>PFLELDTNLPANRVPAGLEKRLCAAAASILGKPADRVNVTVRPGLAMALSGSTEPCAQLSISSIGVVGTAEDNRSHSAHF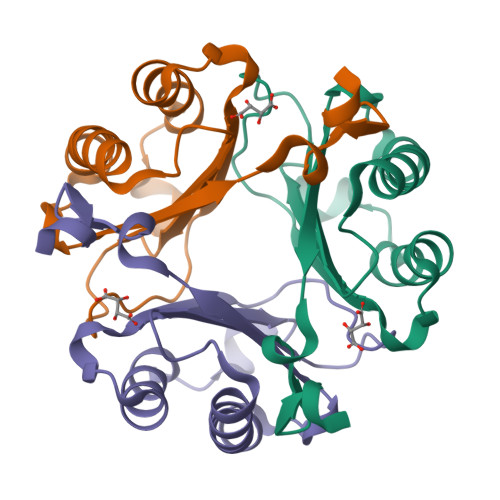FEFLTKELALGQDRILIRFFPLESWQIGKIGTVMTFL[3x]> SDE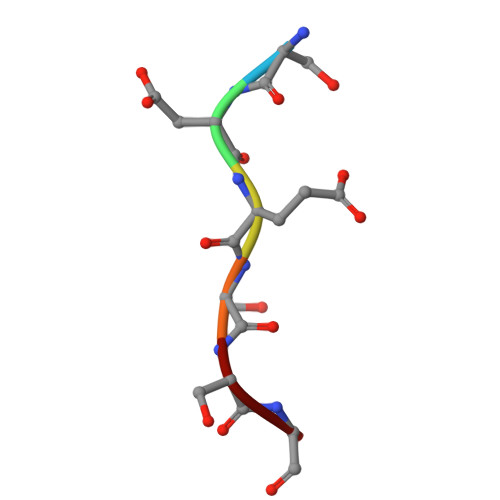SSG N-[(benzyloxy)carbonyl]-L-tyrosyl-D-alanine | C20 H22 N2 O6 | 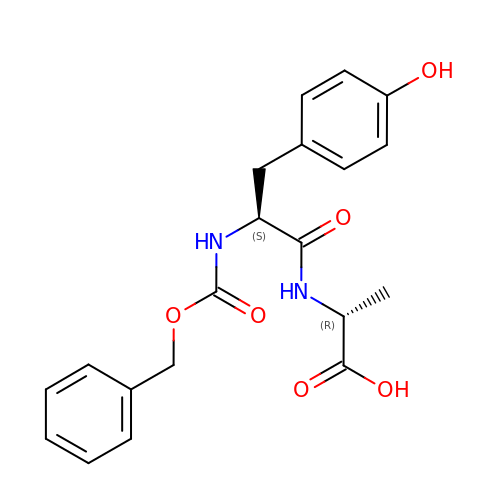LKRYTYVDKGHSPS-DYVFJYSZSA-N>[2x]MNDIAHNLAQVRDKISAAATRCGRSPEEITLLAVSKTAPASAIAEAIDAGQRQFGENYVQEGVDKIRHFQELGVTGLEWHFIGPLQSNKSRLVAEHFDWCHTIDRLRIATRLNDQRPAELPPLNVLIQINISDENSASGIQLAELDELAAAVAELPRLRLRGLMAIPAPESEYVRQFEVARQMAVAFAGLKTRYPHIDTLSLGMSDDMEAAIAAGSTMVRIGTAIFGARDYSAA

The pyridoxal 5′‐phosphate (PLP) homeostasis protein (PLPHP) is a ubiquitous member of the COG0325 family with apparently no catalytic activity. Although the actual cellular role of this protein is unknown, it has been observed that mutations of the PLPHP encoding gene affect the activity of PLP‐dependent enzymes, B6 vitamers and amino acid levels. Here we report a detailed characterization of the Escherichia coli ortholog of PLPHP (YggS) with respect to its PLP binding and transfer properties, stability, and structure. YggS binds PLP very tightly and is able to slowly transfer it to a model PLP‐dependent enzyme, serine hydroxymethyltransferase.

We serendipitously discovered that the K36A variant of YggS, affecting the lysine residue that binds PLP at the active site, is able to bind PLP covalently. This observation led us to recognize that a number of lysine residues, located at the entrance of the active site, can replace Lys36 in its PLP binding role.> MWDVIVVGGGPSGLSAALFLARAGLKVL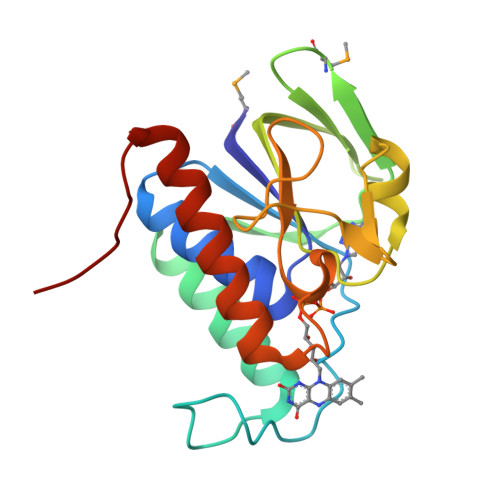VLDGGRSKVKGVSRVPNYPGLLDEPSGEELLRRLEAHARRYGAEVRPGVVKGVRDMGGVFEVETEEGVEKAERLLLCTHKDPTLPSLLGLTRRGAYIDTDEGGRTSYPRVYAAGVARGKVPGHAIISAGDGAYVAVHLVSDLRGEPYKDHAL>[9x]MNNQKVVAVLLQECKQVLDQLLLEAPDVSEEDKSEDQRCRALLPSELRTLIQEAKEMKWPFVPEKWQYKQAVGPEDKTNLKDVIGAGLQQLLASLRASILARDCAAAAAIVFLVDRFLYGLDVSGKLLQVAKGLHKLQPATPIAPQVVIRQARISVNSGKLLKAEYILSSLISNNGATGTWLYRNESDKVLVQSVCIQIR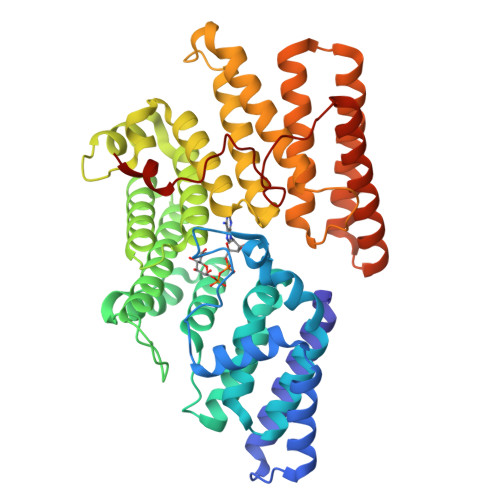GQILQKLGMWYEAAELIWASIVGYLALPQPDKKGLSTSLGILADIFVSMSKNDYEKFKNNPQINLSLLKEFDHHLLSAAEACKLAAAFSAYTPLFVLTAVNIRGTCLLSYSSSNDCPPELKNLHLCEAKEAFEIGLLTKRDDEPVTGKQELHSFVKAAFGLTTVHRRLHGETGTVHAASQLCKEAMGKLYNFSTSSRSQDREALSQEVMSVIAQVKEHLQVQSFSNVDDRSYVPESFECRLDKLIL>GPHMEDENILRNAVNLQVLKFHYPEIESIIDIASHVAVYQFDVGSQKWLKTSIEGTFFLVKDQRARVGYVILNRNSPENLYLFINHPSNVHLVDRYLIHRTENQHVVGLWMFDPNDMSRIFNIVKESLLR[2x];>[2x]MSFTNATFSQVLDDLSARFILNLPAEEQSSVERLCFQIEQAHWFYEDFIRAQNDQLPSLGLRVFSAKLFAHCPLLWKWSKVHEEAFDDFLRYKTRIPVRGAIMLDMSMQQCVLVKGWKASSGWGFPKGKIDKDESDVDCAIREVYEETGFDCSSRINPNEFIDMTIRGQN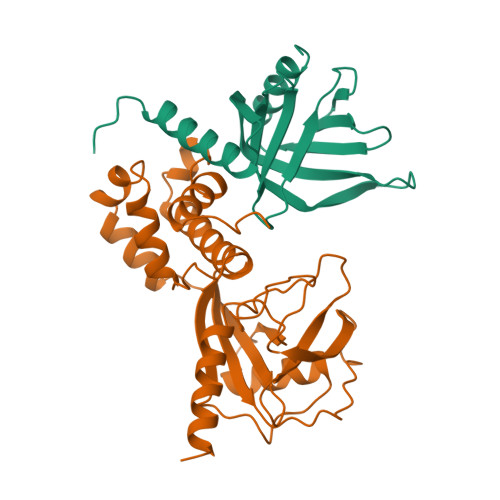VRLYIIPGISLDTRFESRTRKEISKIEWHNLMDLPTFKKNKPQTMKNKFYMVIPFLAPLKKWIKKRNIANNT> GSGANGAKKNWVIKEDPALYKQQGGEYPYYSSFTIALQKLNISHYDSIIDMDNFISKWAEIGRNMKPAARDISHDKFIEVQKTLGKIDAEWSGYHSADVNETFRGDTPVISNSYSWLAEFINESEGKSDTVQKS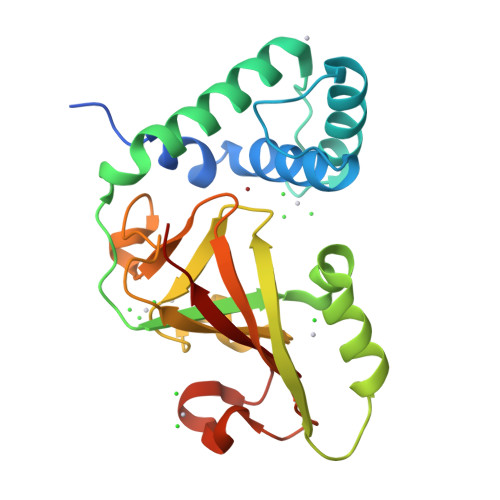MDLEIKSPLIMSTAKDPKMGYVSGKTIMWHFDLEPGHAGVSEGLYASEGEVTFPLYNRMKITSLQYLPEGRSYMDNPEQYGTSHRYIIKARMLPRS3-(2-hydroxy-2,2-diphosphonoethyl)-1-methylpyridinium 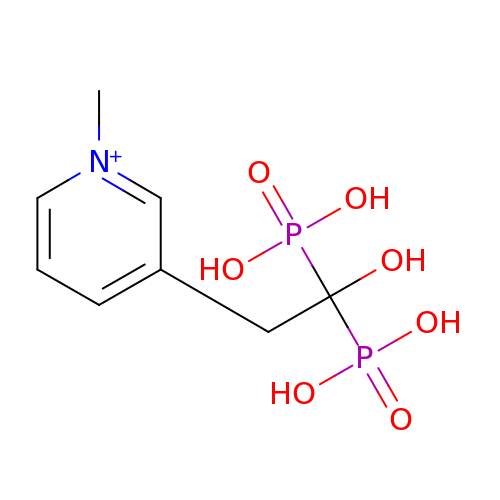| C8 H14 N O7 P2 | BBNRLGQPSIXFHZ-UHFFFAOYSA-O>[8x]GS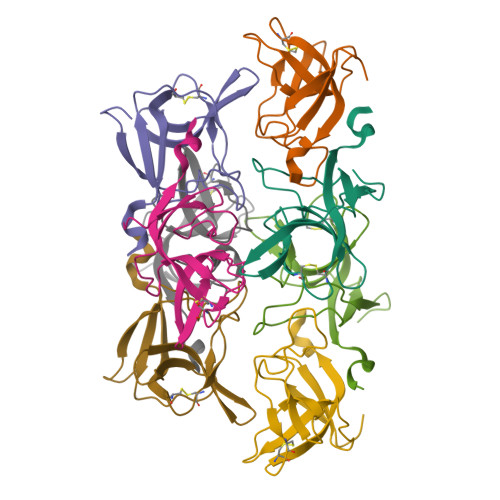HMTTKKASDSAFWLEVEGNSMTAPTGSKPSFPDGMLILVDPEQAVEPGDFCIARLGGDEFTFKKLIRDSGQVFLQPLNPQYPMIPCNESCSVVGKVIASQWPEETFG>MKGSPLFHGLAPEEVDLALSYFQRRLYPQGKPIFYQGDLGQALYLVASGKVRLFRTHLGGQERTLALLGPGELFGEMSLLDEGERSASAVAVEDTELLALFREDYLALIRRLPLVAHNLAALLARRLREADLELDLLSFEEARNRVAYALLKLLRQGLGPLFQIRHHELAALAGT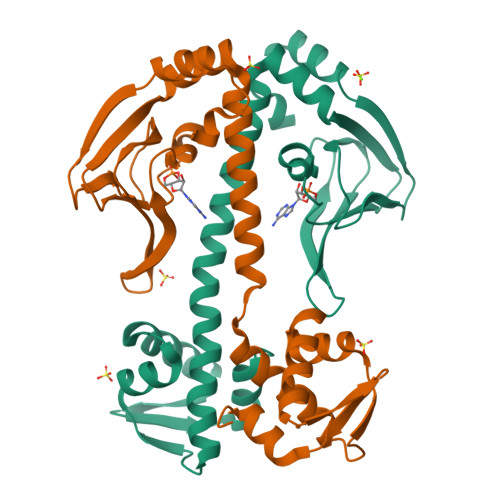SRETVSRVLHALAEEGVVRLGPGTVEVREAALLEEIAFGLA[2x]>[2x]MSLATTHLDVCAVVPAAGFGRRMQTECPKQYLSIGNQTILEHSVHALLAHPRVKRVVIAISPGDSRF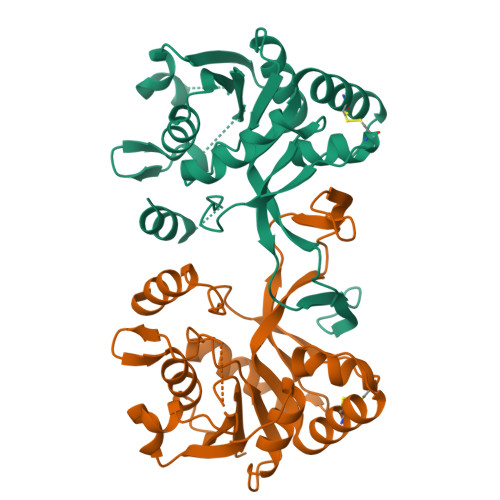AQLPLANHPQITVVDGGDERADSVLAGLKAAGDAQWVLVHDAARPCLHQDDLARLLALSETSRTGGILAAPVRDTMKRAEPGKNAIAHTVDRNGLWHALTPQFFPRELLHDCLTRALNEGATITDEASALEYCGFHPQLVEGRADNIKVTRPEDLALAEFYLTRTIHQENT>MVRASSRLAHPRTTRMSGIEMADTKELQEKFWKALKSDRTVMLGLDGVEDGHARPMTAQIEGDSGGPIWFFT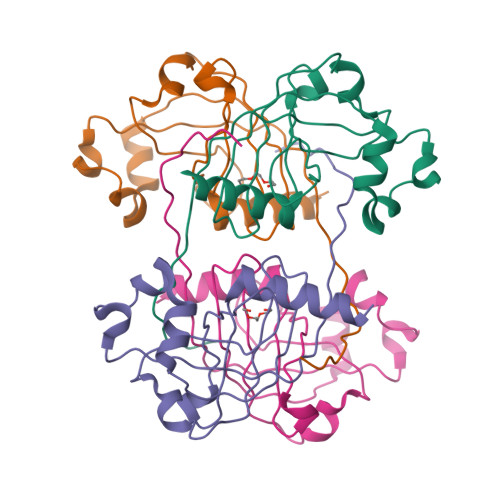SKDNALIAMLGQGRRVIGAFSSKGHDLFASISGSLREDTDPAMVDRLWNPYVAAWYEGGKTDPNLALLRLDADHAQIWLNESSLLAGIKVLLGVDPKKDYQDKVADVPLR[4x]FliL, a component protein of the flagellar motor, is known to enhance the motor performance under high-load conditions in some bacteria. A flagellar protein, FliL, which is a single-transmembrane protein with a large periplasmic region and associates with the flagellar basal body, has been found to be important for the function of the motor under high-load conditions, such as the highly viscous environments in some species. Polar FliL is composed of an N-terminal short cytoplasmic region (residues 1 to 17), a single transmembrane region (TM) (residues 18 to 40), and a periplasmic region (FliLPeri) (residues 41 to 167). FliLPeri shows a remarkable structural similarity to the stomatin/prohibitin/flotillin/HflK/C (SPFH) domain of stomatin family proteins, some of which are involved in modulation of ion channel activities in various organisms.

The FliLPeri crystal belongs to the space group of P42212 and contains 20 molecules in an asymmetric unit. FliLPeri is 17 residues longer at its N terminus than FliLC, but these residues are invisible in the electron density map of FliLPeri. Therefore, we determined the structure of FliLPeri with the same region as that of FliLC. FliLPeri forms a head-to-head stack of two decameric rings in the crystal asymmetric unit. FliLPeri forms a ring assembly in the crystal with an inner diameter of around 8 nm, which is comparable to the size of the stator unit. The bean-shaped subunits are vertically arranged in a parallel manner in the ring. The N terminus locates near the ring-to-ring interface and points toward the outer side of the ring. The C terminus of each subunit is arranged on the inner surface of the ring on the opposite side of the ring-to-ring interface. The side-by-side subunit interaction in the ring is primarily hydrophobic. The subunit interface is formed by characteristic hydrophobic belts on both sides of the subunit along the longitudinal direction of the molecule.

>[20x]HMGSDEPAQAEASQQVQAKASDASPIAYVNLPQAFVFNVTGDSRDRLVQIKAQLMVRGAENEELARYHSPLIESSLLSTFASATVDQLRSPTGRVELRDRASEDIKAALNAAVGKPVIEKVLFTDFVIQ methyl dihydrogen 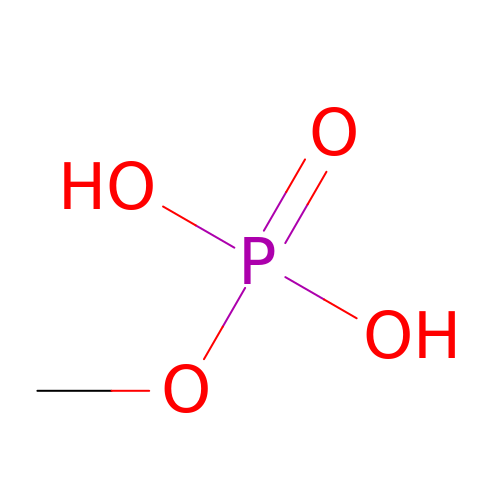phosphate | C H5 O4 P | CAAULPUQFIIOTL-UHFFFAOYSA-N> MSEGFSSSSIQELYQSLKEITNNADVELFEDRITKLDFESTDEPKHANDIIKDRFLRPSNALPWSLLDMVQDVPHTSSPEDCSGKLDYKELLKVPDPINRTSYQFKRTGLEGKISGYKEEVDLKEVANANASNSLSITRSINHNQNSVRGSTAQLPFTPGGIPMKSVKTDSEQNGSSTMANATKLLHKDGQGLFDIPEGMNRGIKPMDSPAENEDQNGQFKELKQLNEIDNELDIRIEANEAKLKEEEKSAKSISEEIMEEATEETTADNADDAEIDELLPIGIDFGRTKPVSKSVPVKKEWAHVVDLNHKIENFDELIPNPARSWPFELDTFQKEAVYHLEQGDSVFVAAHTSAGKTVVAEYAIAMAHRNMTKTIYTSPIKALSNQKFRDFKETFDDVNIGLITGDVQINPDANCLIMTTEILRSMLYRGADLIRDVEFVIFDEVHYVNDQDRGVVWEEVIIMLPQHVKFILLSATVPNTYEFANWIGRTKQKNIYVISTPKRPVPLEINIWAKKELIPVINQNSEFLEANFRKHKEILNGESAKGAPSKTDNGRGGSTARGGRGGSNTRDGRGGRGNSTRGGANRGGSRGAGAIGSNKRKFFTQDGPSKKTWPEIVNYLRKRELLPMVVFVFSKKRCEEYADWLEGINFCNNKEKSQIHMFIEKSITRLKKEDRDLPQILKTRSLLERGIAVHHGGLLPIVKELIEILFSKGFIKVLFATETFAMGLNLPTRTVIFSSIRKHDGNGLRELTPGEFTQMAGRAGRRGLDSTGTVIVMAYNSPLSIATFKEVTMGVPTRLQSQFRLTYNMILNLLRIEALRVEEMIKYSFSENAKETLQPEHEKQIKVLQEELQTIEYKSCEICDNDIEKFLELMLAYKEATVNLMQEMVKSPSILHILKEGRLVAFRDPNDCLKLGFVFKVSLKDAVCVIMTFTKPYKLPNGEPNHLIYFPKADGYRRRNFPKFQKTDFYMEEVPVTAIEVITKRKFAAPLGKVIKKDVAALNEFNAETNNILDGKTLKEAINIEKQGLKIHQILL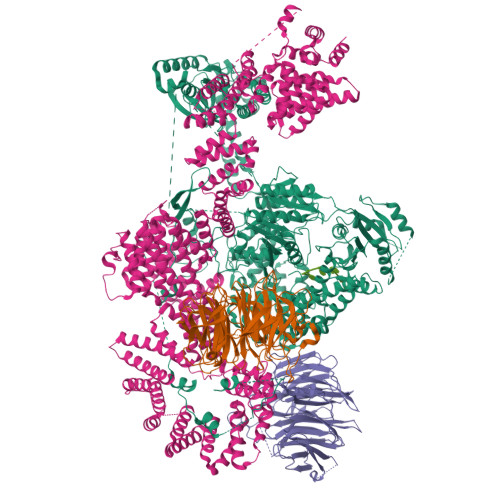DRTNIRDEIFKLKSIKCPNLSQHIVPKFKAHVIKKKIEELYHLMSDQNLSLLPDYEKRLAVLKDTEFIDQNHNVLLKGRVACEINSGYELVLTELILDNFLGSFEPEEIVALLSVFVYEGKTREEEPPIVTPRLAKGKQRIEEIYKKMLCVFNTHQIPLTQDEAEFLDRKRFAMMNVVYEWARGLSFKEIMEMSPEAEGTVVRVITWLDEICREVKTASIIIGNSTLHMKMSRAQELIKRDIVFAASLYL;>[2x]MSKVFIATANAGKAHDADIFSVSACNSFTVSCSGDGYLKVWDNKLLDNENPKDKSYSHFVHKSGLHHVDVLQAIERDAFELCLVATTSFSGDLLFYRITREDETKKVIFEKLDLLDSDMKKHSFWALKWGASNDRLLSHRLVATDVKGTTYIWKFHPFADESNSLTLNWSPTLELQGTVESPMTPSQFATSVDISERGLIATGFNNGTVQISELSTLRPLYNFESQHSMINNSNSIRSVKFSPQGSLLAIAHDSNSFGCITLYETEFGERIGSLSVPTHSSQASLGEFAHSSWVMSLSFNDSGETLCSAGWDGKLRFWDVKTKERITTLNMHCDDIEIEEDILAVDEHGDSLAEPGVFDVKFLKKGWRSGMGADLNESLCCVCLDRSIRWFREAGGK;> GPDSMSDIKQLLKEAKQELTNRDYEETIEISEKVLKLDPDNYFAHIFLGKALSSLPASNNVSSNRNLERATNHYVSAAKLVPDNLLAWKGLFLLFRTTEVVPDILSYDEYFDLCGQYADALLKQEQSQVELINDIKLLKKTHPDCQKAFYQHLKPGSLMAETIGRHLSTPQDALLNLIKILSNIETTEIGKTLSQNRLKLKASDPDYQIKLNSFSWEIIKNSEIDQLYNQLVNILADDQKRSEIENQWLEYRIKVLKSMPLDVKKDFFTKVKEMVEDMVLVNHQSLLAWQKYFEWTDYEDLDNMDAPLIIKYFKKFPKDPLAMILYSWLSSKLSKYDIKSLESANKPPEGHKKTEKETDIKDVDETNEDEVKDRVEDEVKDRVEDEVKDQDEEAKEDEEEDLDDIEIGLLEEEVVTVLTENIVKCKNNILAHRILCQYYLLTKEYEAALPYIKNGISLIAYNIKDLGVHLPLTKREFSLDLATVYTYVDAPKDHNAALKLYDNILSGDFSNIQAKMGKGIIFIERKNWKDAMTLLTQVHEQSPNNLEVLSELSWSKAHMGYMDEALAGLDTVIKGIKGMDLRSIDFRALNLWRQAKVYIMKHASINDAKQENVKCAFKLLIQSIKILDTFAPGFSTLGDIYCHYYKDHLRAFKCYFKAFDLDAGDYTAAKYITETYASKPNWQAASSIASRLIKGEKAKAELRSNNWPFRVVGIAHLEKQEESDSIEWFQSALRVDPNDVESWVGLGQAYHACGRIEASIKVFDKAIQLRPSHTFAQYFKAISLCDVGEYLESLDILEKVCQEAATEESFQIGLVEVLMRCSLDLYSQGFLLKSVSIAKDTIERIKIIISELKCENQQVWIYLSQVLRLFIWIESKVDTLPVESLVSIFENSQFSGSEEIDSVDNIKIDTLLDSTTDDNVSIACKFLILASKYSVSDQKFTDIAGTVRASYWYNIGISELTAFITLKEPQYRDAAIFAFKKSIQLQSNTSETWIGLGIATMDINFRVSQHCFIKATALEPKATNTWFNLAMLGLKKKDTEFAQQVLNKLQSLAPQDSSPWLGMALILEEQGDIIGSSKLFAHSFILSNGRSKAAQFMYAKNVLENHINNGDDERDIETVEKLTTASIALEQFFKKSPDSQFALQCALLTLERLHHYENANELANRLIGILEKKFEKTQDERELFNFAIIKGQFARIHLGLGNFELSIENADLSQGIISESSDEKSMKTKISNHICLGLSYFFLNDFDQTLNQFQELLSISKDSKHLVVLIAKVLYDVGESDTKEIALQELTEYIATSGADLLVTLTIAAMSILDDKREDLSIILEELKALPLSKQIIDKHKDAPYLIEEITKRLYRNDTGKQVWQRSAYFFPNNLKVWERLDKNIQRRIASNGQNKVTAEEMSKLYCESKNLRSIQRGMFLCPWNVTAVKALNECF>[4x]SMYKVRDISLAEWGRRE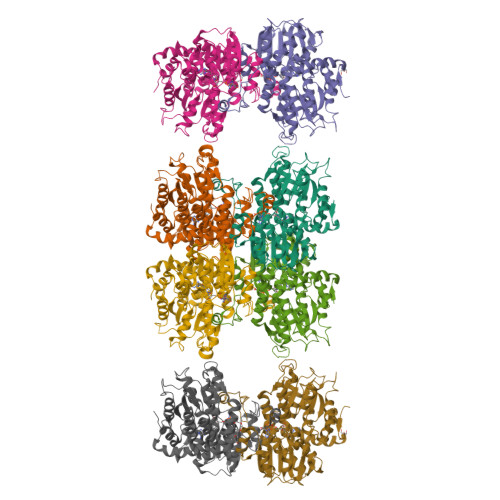LELAENEMPGLMELRREYGPSKPLKGAKIAGCLHMTMQTAVLIETLVELGAEVRWASCNIFSTQDHAAAAIAKRGIPVFAWKGETEEEYMWCMKQTLKGFSGDGYPNMLLDDGGDLTNYVLDECKELDGKIYGVSEETTTGVKNLYKRLQRGKLTIPAMNVNDSVTKSKFDNLYGCRESLVDGIKRATDVMIAGKTACVCGYGDVGKGCAAALRGFGARVVVTEVDPINALQAAMEGYQVLLVEDVVEEAHIFVTTTGNDDIITSEHFPRMRDDAIVCNIGHFDTEIQVAWLKANAKERVEVKPQVDRYTMANGRHIILLAEGRLVNLGCASGHPSFVMSNSFCNQVLAQIELWTNRDTGKYPRGAKAQVYFLPKKLDEKVAALHLGKLGAKLTKLTPKQAEYINCPVDGPFKPDHYRY>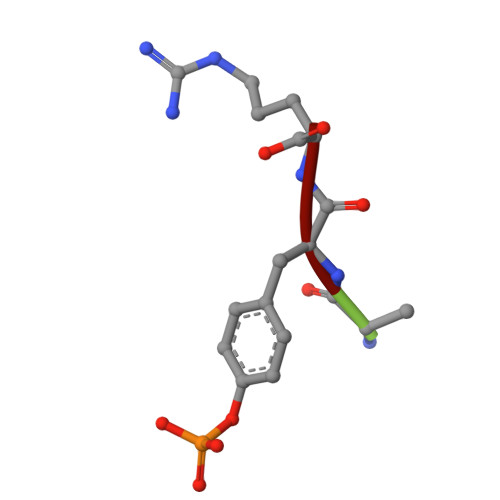 AYR>GMSQLDKDAFEVLLANCADEPIQFPGAIQPHGLLFTLKEPELTILQVSANVQSVLGKVPDQLAGQTLDCVLGAGWAEVIRSTSANDSLVDVPRLLMSVEGVEFEALLHRSQEALVLELEIQDKAAQAISYSERTGNMGRMLRQLHAAADLQTLYEVSVREIQRMTGYDRVLIYRFEEEGHGQVIAEASAPAMELFNGLFFPASDIPEQARELYRRNWLRIIPDANYTPVPLVPQLRPDTQQQLDLSFSTLRSVSPIHCQYMKNMGVLSSMSVSLIQGGKLWGLISCGHRTPLYVSHELRSACQAIGQVLSLQISAMEALEVSRQRETKIQTLQQLHQMMATSDTDVFDGLAQQPQLLMDLVGATGVAIIEDRQTHCYGNCPEPSDIRALHTWMMAGGEPVYASHHLSSVYPPGEAYQTLASGVLAMSLPKPVDNGVIWFRPEVKQSVQWSGDPNKPLNLDASDNTLRLQPRTS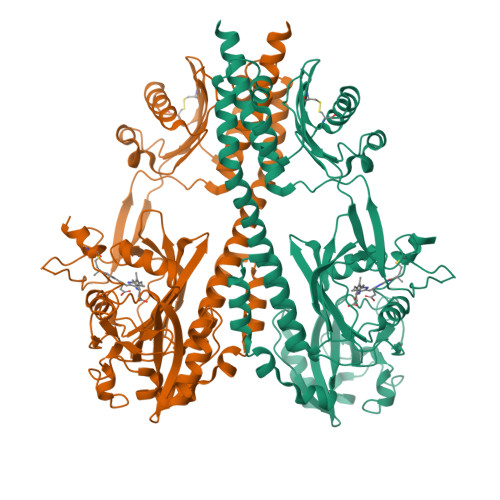FEIWKVEMTGIATKWSHGDVFAANDLRRSALENDLARQVSKEQQAVRARDELVAVVSHDLRNPMTVISMLCGMMQKSFSSDGPHTSRRISTAIDTMQQAASRMNVLLEDLLDTSKIEAGRYTITPQPLEVSQIFEEAYTLLAPLAMDKSIEISFNAEPDIKVNADPERLFQVLSNLIGNAIKFTPKLGRIGVAAMSNGDEVVFTVRDSGEGIPPEQLPHIFERYWTVKEGNPTGTGLGLYISQGIIKAHGGELAAQSQVGHGSEFRFTVPIAH[2x]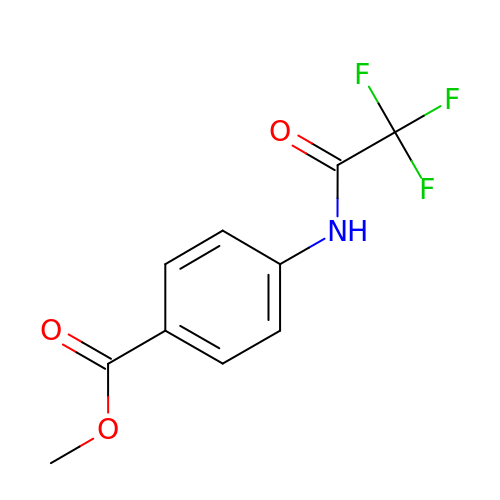methyl 4-[(trifluoroacetyl)amino]benzoate | C10 H8 F3 N O3 | MDDVOSSRTNAXHJ-UHFFFAOYSA-N>GAMGSGAMGSQQFPQFHVKSGLQIKKNAIIDDYKVTSQVLGLGINGKVLQIFNKRTQEKFALKMLQDCPKARREVELHWRASQCPHIVRIVDVYENLYAGRKCLLIVMECLDGGELFSRIQDRGDQAFTEREASEIMKSIGEAIQYLHSINIAHRDVKPENLLYTSKRPNAILKLTDFGFAKETTSHNSLTTPCYTPYYVAPEVLGPEKYDKSCDMWSL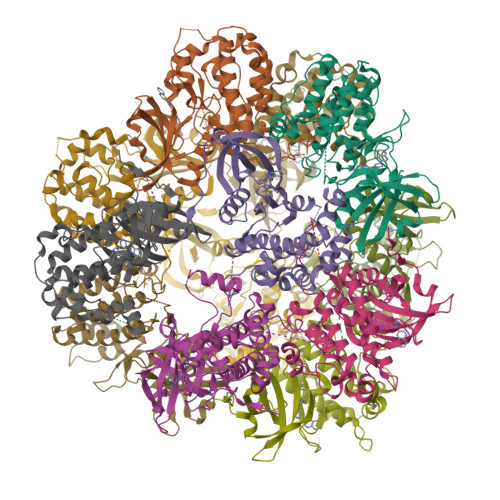GVIMYILLCGYPPFYSNHGLAISPGMKTRIRMGQYEFPNPEWSEVSEEVKMLIRNLLKTEPTQRMTITEFMNHPWIMQSTKVPQTPLHTSRVLKEDKERWEDVKEEMTSALATMR[12x]>[4x]MGSSHHHHHHSQDPMSNRLKNEVIAITGGGAGIGLAIASAALREGAKVALIDLDQGLAERSAAMLSTGGAVAKGFGADVTKAADITAAITSAEQTIGSLTGLVNNAGIAGFGSVHDADAAAWDRIMAVNVTGTFLASKAALAGMLERHKGTIVNFGSVAGLVGIPTMAAYCAAKGAIVNLTRQMAADYSGRG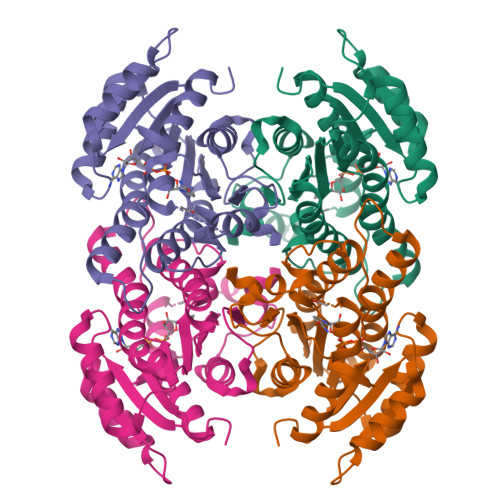VRVNAVCPGTVTSTGMGQQLLGSDTSPEVQARRLAKYPIGRFGTPEDIAEAVIFLLSDQAAFVTGAAFAVDGGMTAI> MTQQPFQLPHFYLPHPARLNPHLDEARAHSTTWAREMGMLEGSGVWEQSDLEAHDYGLLCAYTHPDCDGPALSLITDWYVWVFFFDDHFLEKYKRSQDRLAGKAHLDRLPLFMPLDDAAGMPEPRNPVEAGLADLWTRTVPAMSADWRRRFAVATEHLLNESMWELSNINEGRVANPVEYIEMRRKVGGAPWSAGLVEYATAEVPAAVAGTRPLRVLMETFSDAVHLRNDLFSYQREVEDEGELSNGVLVLETFFGCTTQEAADLVNDVLTSRLHQFEHTAFTEVPAVALEKGLTPLEVAAVGAYTKGLQDWQSGGHEWHMR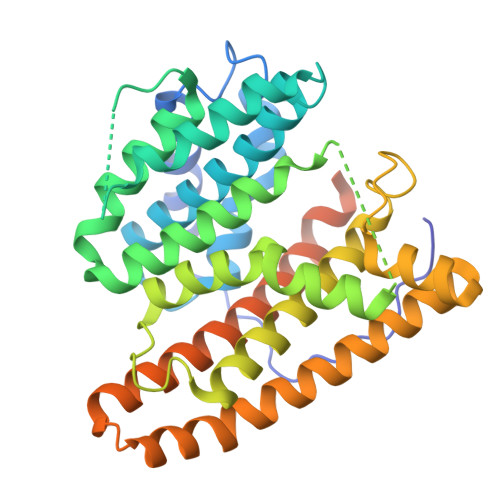SSRYMNKGERPLAGWQALTGPGTSAADVGALLADAVAQRARSYT> MVTRMATKVSLEGKRVVLVPYMAEHVPKYHQWMQDSALLEATGSEPLSLEQEYEMQLSWTQDPNKRTFIVLDKDFVKGDLAHGQPHVEAMTGDVNIYMNDVDDPKVAEVEIM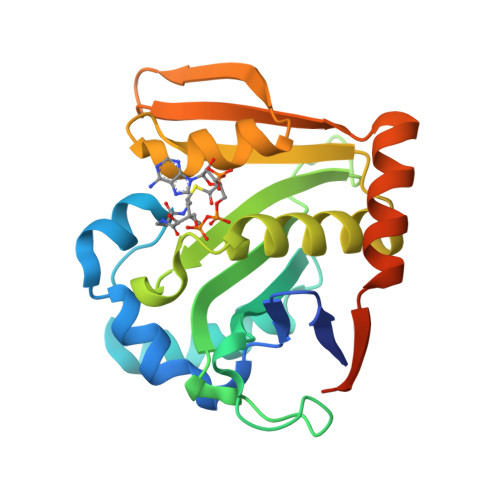IAEPRSRGKGLGKESVLIMMAYGVKNLEIHKFTAKIGESNTASLSLFRKLGFEESSYSGIFKEVTLEYPVTNLRREELLKLLDEVIRHTHSSNNPSDSLLSGEATA> MKFAEHLSAHITPEWRKQYIQYEAFKDMLYSAQDQAPSVEVTDEDTVKRYFAKFEEKFFQTCEKELAKINTFYSEKLAEAQRRFATLQNELQSSLDAQKESTGVTTLRQRRKPVFHLSHEERVQHRNIKDLKLAFSEFYLSLILLQNYQNLNFTGFRKILKKHDKILETSRGADWRVAHVEVAPFYTCKKINQLISETEAVVTNELEDGDRQKAMKRLRVPPLGAAQPAPAWTTFRVGLFCGIFIVLNITLVLAAVFKLETDRSIWPLIRIYRGGFLLIEFLFLLGINTYGWRQAGVNHVLIFELNPRSNLSHQHLFEIAGFLGILWCLSLLACFFAPISVIPTYVYPLALYGFMVFFLINPTKTFYYKSRFWLLKLLFRVFTAPFHKVGFADFWLADQLNSLSVILMDLEYMICFYSLELKWDESKGLLPNNSEESGICHK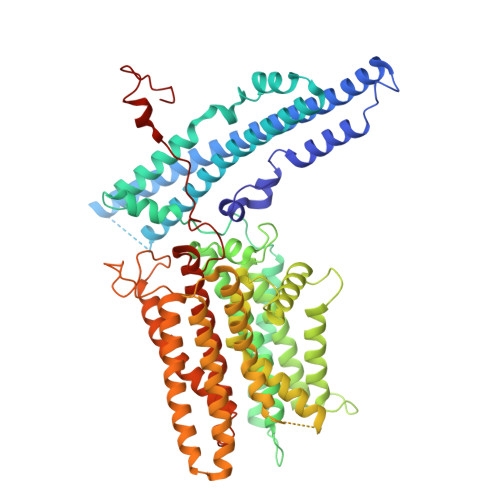YTYGVRAIVQCIPAWLRFIQCLRRYRDTKRAFPHLVNAGKYSTTFFMVTFAALYSTHKERGHSDTMVFFYLWIVFYIISSCYTLIWDLKMDWGLFDKNAGENTFLREEIVYPQKAYYYCAIIEDVILRFAWTIQISITSTTLLPHSGDIIATVFAPLEVFRRFVWNFFRLENEHLNNCGEFRAVRDISVAPLNADDQTLLEQMMDQDDGVRNR4-{[(4R)-6-fluoro-3,4-dihydro-2H-1-benzopyran-4-yl]sulfamoyl}-2,5-dimethylfuran-3-carboxylic acid | C16 H16 F N O6 S | 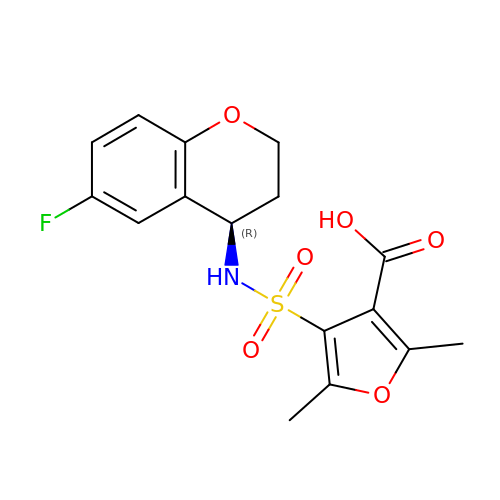YXLDXDUEWBKCKU-GFCCVEGCSA-N> AGEQLNEFSSSGLGRAYSGEGAIADDAGNVSRNPALITMFDRPTFSAGAVYIDPDVNISGTSPSGRSLKADNIAPTAWVPNMHFVAPINDQFGWGASITSNYGLATEFNDTYAGGSVGGTTDLET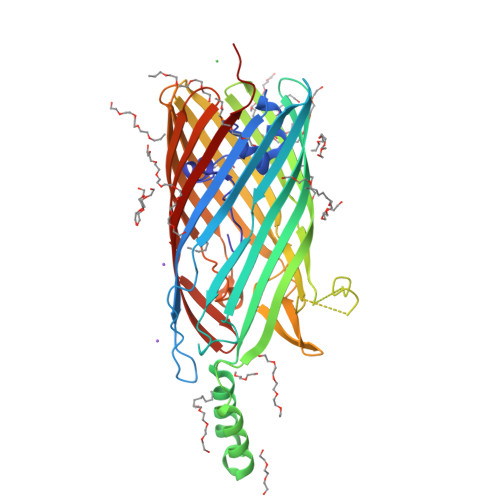MNLNLSGAYRLNNAWSFGLGFNAVYARAKIERFAGDLGQLVAGQIMQSPAGQTQQGQALAATANGIDSNTKIAHLNGNQWGFGWNAGILYELDKNNRYALTYRSEVKIDFKGNYSSDLNRAFNNYGLPIPTATGGATQSGYLTLNLPEMWEVSGYNRVDPQWAIHYSLAYTSWSQFQQLKATSTSGDTLFQKHEGFKDAYRIALGTTYYYDDNWTFRTGIAFDDSPVPAQNRSISIPDQDRFWLSAGTTYAFNKDASVDVGVSYMHGQSVKINEGPYQFESEGKAWLFGTNFNYAFHHHHHH> MVNETSGRENTPKGQPGSIWLREVKQRPARQPLSREQIVQAAVRLLDEG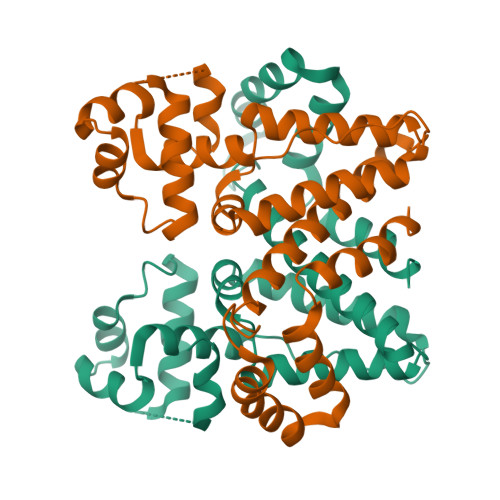GVRNLRMRQLADSLNSAPMSLYWHVSTKDDLLELAIDAVFPDPPSRSGTGDWRDDIKAGATDLFEVLLRHSWMIELMGGHPPVGPRALAHTSAIIEILEQAHFSPRQLDSALSAIYYYTVGAALSEASWQAMARQSAESEEEWVSRLGPYLGMATQSHPASLADYVKRSASSSTGQRFHDGLECMVSGMGQMRSQDSLEHHHHHH>GAGSMGSLEKFNLIDEPWIPVLKGGRVVEVGIGEALLRAHEFARIETPSPLEEAVLHRLLLAVLHRALSGPRCPEDVLDWWRKGGFPQDPIRDYLNRFRDRFFLFHPEAPFLQVADLPEENPLPWSKLLPELASGNNPTLFDHTTEENLPKATYAQAARALLVHQAFAPGGLLRRYGVGSAKDAPVARPALFLPTGQNLLETLLLNLVPYTPEDDAPIWEVPPLRLGDLEGARTKWPLTGRTRVYTWPARGVRLLDEGDGVRFMGYGPGVEPLEATHRDPMVAQRLDAKGNLLVLRLSEERSFWRDFSAMLPRQGGKVAATLEHAENLQGELEDEGLEGRITLRVLGQVSDQ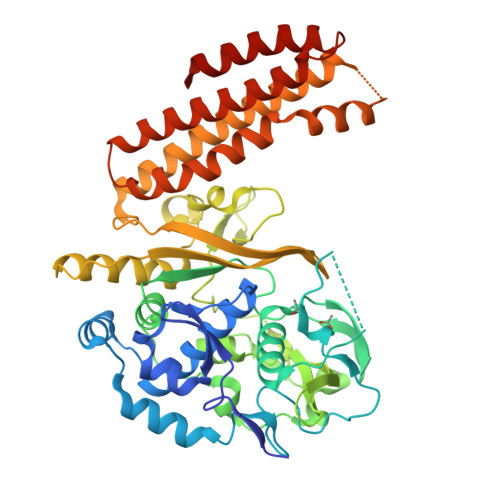AKVLDIRREVYPLPSGLLTPKAEENLEKALKMAEELGQGLKHLAQEVAKAVVGERDRGHGRSPYLEELTKLANSLPLERLYWHALDGAFPRFFARVEEEASLDLWREALRGAALEAWKATRRFLGTGARHLKALAQGEQEFGRLLGELGEEVRT[2x]>[6x]MKSVMTTTISAADAAGRFPSSSDLESVQGNIQRAAARLEAAEKLASNHEAVVKEGGDA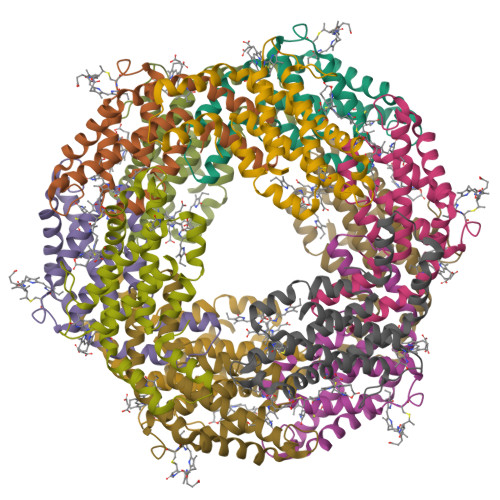CFAKYSYLKNPGEAGDSQEKVNKCYRDVDHYMRLVNYSLVVGGTGPLDEWAIAGAREVYRTLNLPSASYVAAFAFTRDRLCVPRDMSAQAGGEYVAALDYIVNALT;>[6x]MLDAFSRVVVNSDAKAAYVGGSDLQALKKFITDGNKRLDSVSFVVSNASCIVSDAVSGMICENPGLIAPGGNCYTNRRMAACLRDGEIILRYASYALLAGDPSVLEDRCLNGLKETYIALGVPTNSSVRAVSIMKASATAFVSGTASDRKMACPDGDCSALASELGSYCDRVAAAIS2-(3-methylphenyl)-5,7-bis(oxidanyl)chromen-4-one 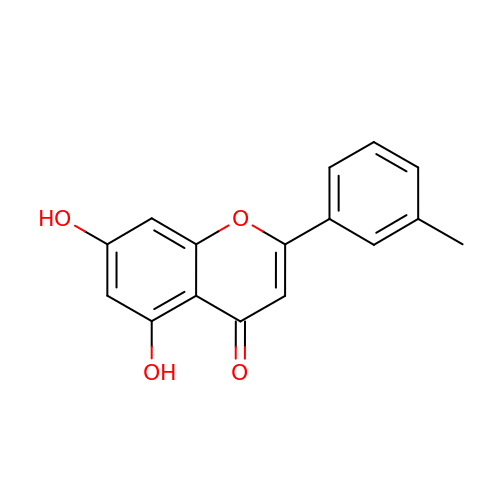| C16 H12 O4 | IGTBSDZAEVYRPZ-UHFFFAOYSA-N> MDAMEVVGTIDHRDREEFRSRGFAILPQVASESEVAWLRQAYDRLFVRRATPGAEDFYDIAGQRDREGPPLLPQIIKPEKYVPELLDSPHFARCRSIASAFLDMAEEELEFYGHAILKPPRYGAPTPWHQDEAYMDPRWRRRGLSIWTTLDEATVESGCLHYLPGGHRGPVLPHHHIDNDDRIRGLMTDDVDPTSAVACPLAPGGAVVHDFRTPHYAGPNLTDQPRRAYVLVFMSAPA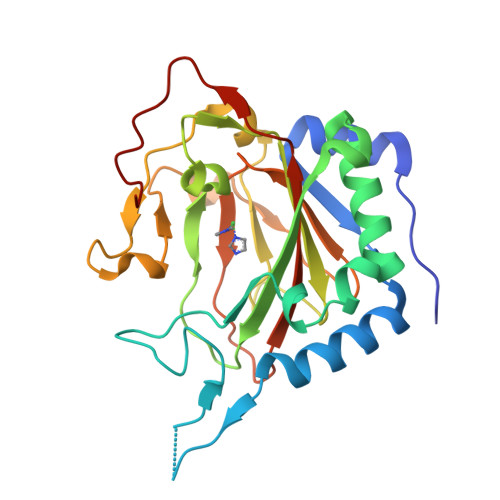EVADPEPRPWMDWG> MLGTGPAAATTAATTSSNVSVLQQFASGLKSRNEETRAKAAKELQHYVTMELREMSQEESTRFYDQLNHHIFELVSSSDANERKGGILAIASLIGVEGGNATRIGRFANYLRNLLPSNDPVVMEMASKAIGRLAMAGDTFTAEYVEFEVKRALEWLGADRNEGRRHAAVLVLRELAISVPTFFFQQVQPFFDNIFVAVWDPKQAIREGAVAALRACLILTTQREPKEMQKPQWYRHTFEEAEKGFDETLAKEKGMNRDGSTSGSGDYKDDDDKGSTSGSGDRIHGALLILNELVRISSMEGERLREEMEEITQQQLVHDKYCKDLMGFGTKPRHITPFTSFQAVQPQQSNALVGLLGYSSHQGLMGFGTSPSPAKSTLVESRCCRDLMEEKFDQVCQWVLKCRNSKNSLIQMTILNLLPRLAAFRPSAFTDTQYLQDTMNHVLSCVKKEKERTAAFQALGLLSVAVRSEFKVYLPRVLDIIRAALPPKDFAHKRQKAMQV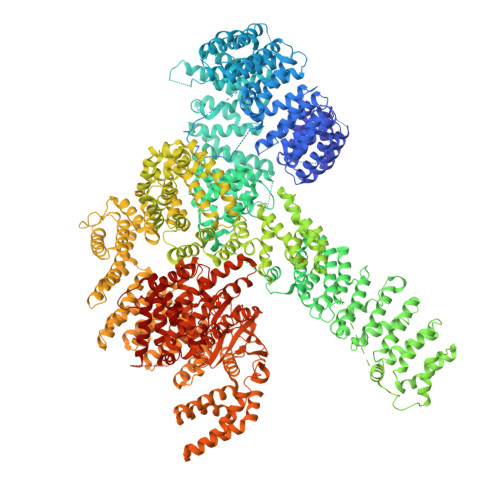DATVFTCISMLARAMGPGIQQDIKELLEPMLAVGLSPALTAVLYDLSRQIPQLKKDIQDGLLKMLSLVLMHKPLRHPGMPKGLAHQLASPGLTTLPEASDVGSITLALRTLGSFEFEGHSLTQFVRHCADHFLNSEHKEIRMEAARTCSRLLTPSIHLISGHAHVVSQTAVQVVADVLSKLLVVGITDPDPDIRYCVLASLDERFDAHLAQAENLQALFVALNDQVFEIRELAICTVGRLSSMNPAFVMPFLRKMLIQILTELEHSGIGRIKEQSARMLGHLVSNAPRLIRPYMEPILKALILKLKDPDPDPNPGVINNVLATIGELAQVSGLEMRKWVDELFIIIMDMLQDSSLLAKRQVALWTLGQLVASTGYVVEPYRKYPTLLEVLLNFLKTEQNQGTRREAIRVLGLLGALDPYKHKVNIGMIDQSRDASAVSLSESKSSQDSSDYSTSEMLVNMGNLPLDEFYPAVSMVALMRIFRDQSLSHHHTMVVQAITFIFKSLGLKCVQFLPQVMPTFLNVIRVCDGAIREFLFQQLGMLVSFVKSHIRPYMDEIVTLMREFWVMNTSIQSTIILLIEQIVVALGGEFKLYLPQLIPHMLRVFMHDNSPGRIVSIKLLAAIQLFGANLDDYLHLLLPPIVKLFDAPEAPLPSRKAALETVDRLTESLDFTDYASRIIHPIVRTLDQSPELRSTAMDTLSSLVFQLGKKYQIFIPMVNKVLVRHRINHQRYDVLICRIVKGYTLADEEEDPLIYQHRMLRSGQGDALASGPVETGPMKKLHVSTINLQKAWGAARRVSKDDWLEWLRRLSLELLKDSSSPSLRSCWALAQAYNPMARDLFNAAFVSCWSELNEDQQDELIRSIELALTSQDIAEVTQTLLNLAEFMEHSDKGPLPLRDDNGIVLLGERAAKCRAYAKALHYKELEFQKGPTPAILESLISINNKLQQPEAAAGVLEYAMKHFGELEIQATWYEKLHEWEDALVAYDKKMDTNKDDPELMLGRMRCLEALGEWGQLHQQCCEKWTLVNDETQAKMARMAAAAAWGLGQWDSMEEYTCMIPRDTHDGAFYRAVLALHQDLFSLAQQCIDKARDLLDAELTAMAGESYSRAYGAMVSCHMLSELEEVIQYKLVPERREIIRQIWWERLQGCQRIVEDWQKILMVRSLVVSPHEDMRTWLKYASLCGKSGRLALAHKTLVLLLGVDPSRQLDHPLPTVHPQVTYAYMKNMWKSARKIDAFQHMQHFVQTMQQQAQHAIATEDQQHKQELHKLMARCFLKLGEWQLNLQGINESTIPKVLQYYSAATEHDRSWYKAWHAWAVMNFEAVLHYKHQNQARDEKKKLRHASGANITNATTAATTAATATTTASTEGSNSESEAESTENSPTPSPLQKKVTEDLSKTLLMYTVPAVQGFFRSISLSRGNNLQDTLRVLTLWFDYGHWPDVNEALVEGVKAIQIDTWLQVIPQLIARIDTPRPLVGRLIHQLLTDIGRYHPQALIYPLTVASKSTTTARHNAANKILKNMCEHSNTLVQQAMMVSEELIRVAILWHEMWHEGLEEASRLYFGERNVKGMFEVLEPLHAMMERGPQTLKETSFNQAYGRDLMEAQEWCRKYMKSGNVKDLTQAWDLYYHVFRRISKQLPQLTSLELQYVSPKLLMCRDLELAVPGTYDPNQPIIRIQSIAPSLQVITSKQRPRKLTLMGSNGHEFVFLLKGHEDLRQDERVMQLFGLVNTLLANDPTSLRKNLSIQRYAVIPLSTNSGLIGWVPHCDTLHALIRDYREKKKILLNIEHRIMLRMAPDYDHLTLMQKVEVFEHAVNNTAGDDLAKLLWLKSPSSEVWFDRRTNYTRSLAVMSMVGYILGLGDRHPSNLMLDRLSGKILHIDFGDCFEVAMTREKFPEKIPFRLTRMLTNAMEVTGLDGNYRITCHTVMEVLREHKDSVMAVLEAFVYDPLLNWRLMDTNTKGNKRSRTRTDSYSAGQSVEILDGVELGEPAHKKTGTTVPESIHSFIGDGLVKPEALNKKAIQIINRVRDKLTGRDFSHDDTLDVPTQVELLIKQATSHENLCQCYIGWCPFW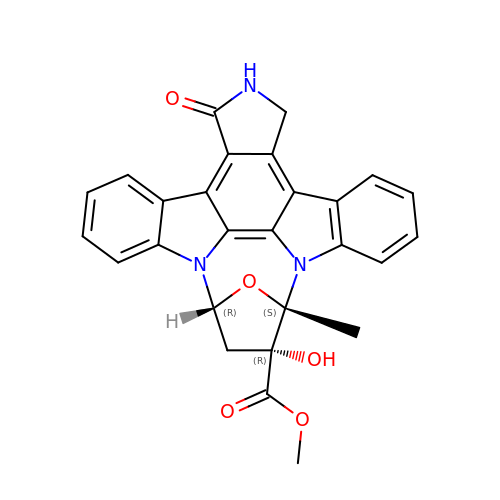K-252A | C27 H21 N3 O5 | KOZFSFOOLUUIGY-SOLYNIJKSA-N> TTLERPQPKLSMADKAARIDAICEKARILPVITIAREEDILPLADALAAGGIRTLEVTLRSQHGLKAIQVLREQRPELCVGAGTVLDRSMFAAVEAAGAQFVVTPGITEDILEAGVDSEIPLLPGIS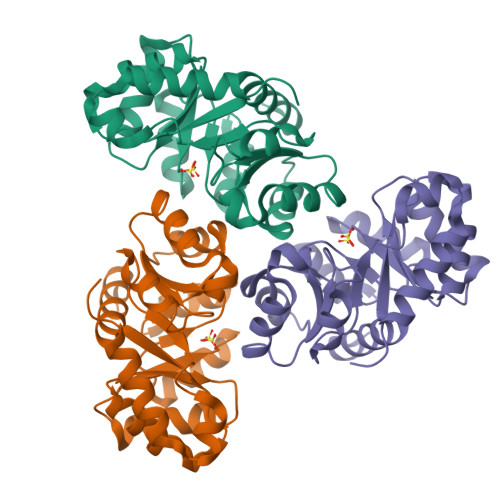TPSEIMMGYALGYRRFKLFPAEISGGVAAIKAFGGPFGDIRFCPTGGVNPANVRNYMALPNVMCVGTTWMLDSSWIKNGDWARIEACSAEAIALLDAN> MVEPQHNVMQMGGDFANNPNAQQFIDKMVNKHGFDRQQLQEILSQAKRLDSVLRLMDNQAPTTSVKPPSGPNGAWLRYRKKFITPDNVQNGVVFWNQYEDALNRAWQVYGVPPEIIVGIIGVETRWGRVMGKTRILDALATLSFNYPRRAEYFSGELETFLLMARDEQDDPLNLKGSFAGAMGYGQFMPSSYKQYAVDFSGDGHINLWDPVDAIGSVANYFKAHGWVKGDQVAVMAN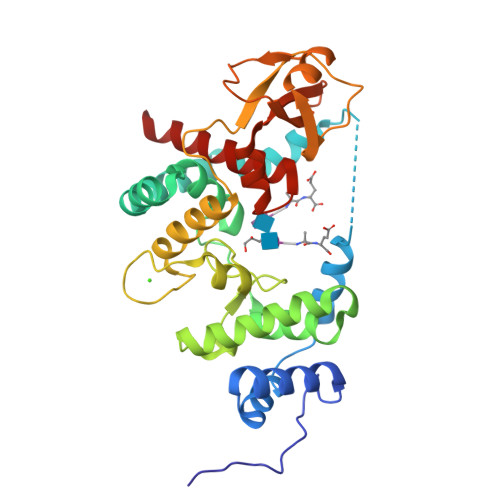GQAPGLPNGFKTKYSISQLAAAGLTPQQPLGNHQQASLLRLDVGTGYQYWYGLPNFYTITRYNHSTHYAMAVWQLGQAVALARVQ> MTLETAFMLPVQDAQHSFRRLLKAMSEPGVIVALHQLKRGWQPLNIATTSVLLTLADNDTPVWLSTPLNNDIVNQSLRFHTNAPLVSQPEQATFAVTDEAISSEQLNALSTGTAVAPEAGATLILQVASLSGGRMLRLTGAGIAEERMIAPRLPECILHELTERPHPFPLGIDLILTCGE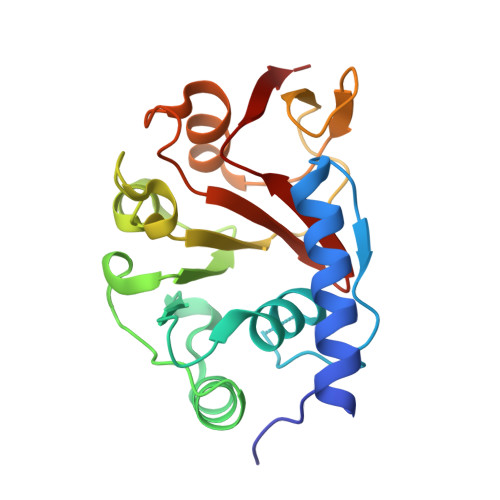RLLAIPRTTHVEVC>[2x]ESEVEQTPLQEALNQLMRQLQRKDPSAFFSFPVTDFIAPGYSMIIKHPMDFSTM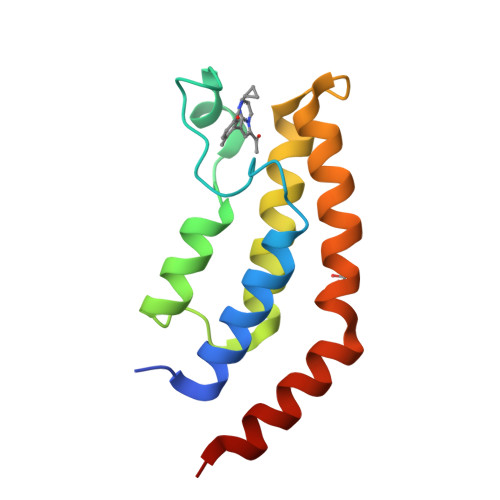KEKIKNNDYQSIEELKDNFKLMCTNAMIYNKPETIYYKAAKKLLHSGMKILSQERIQSLKQSIDFMADL> ETGQTLAANIWSDKTTAQNEPINLTNANAPIKNAKNLNSTITNVAAFDTKLNHLLVDTITGRVFVGGVNRLYQLSPDLELSETVKTGPQNDSVECSILDCPLNAVRSPTDNYNKVLLIDRATSRLIACGSLFQGTCTVRNLQNVSIIEHEVPDAVVANDANSSTVAFIAPGPPQHPVTNVMYVGVTYTNNSPYRSEIPAVASRSLEKTKMFQIASSAVTTGTRTFINSYARETYFVNYVYGFSSERFSYFLTTQLKHSHHSSPKEYITKLVRICQEDSNYYSYTEIPVECISDAQGGTKFNLVQAGFLGKPSSDLAQSLGISIQDDVLFAVFSKGEGNTPTNNSALCIYSLKSIRRKFMQNIKSCFNGSGMRGLDFISPSMPCVLTKLQTIGEDFCGLDVNSPLGGETPITSVPVAMFNTKLTSVAATSTSGYTVVFVGTSDGFLKKVVIESSSIANEYASFAVDLGSEINRDMQFDNQNLYIYVMSKTKVSKVKVFDCSDYKTCGDCLGARDPYCGWCSLENKCSPRSNCQDDANDPLYWVSYKTGKCTTITSVVPHQLQRTTARTLELIIDHLPQLKENLICAFTTEDKALFTNATKKRNGVNCTTPRTDMLPQIEQGKHHFTAKLSVRTRNGPDLVSTDFTFFDCSTHSSC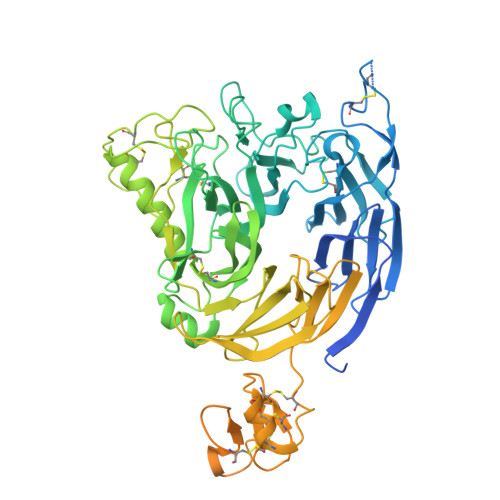TRCVSSEFPCDWCVEAHRCTHDTAENCRNDILVTGVSRIGPSYRSGPGFCPTGTKHHHHHH> MAETRVIVVGNEKGGAGKSTIAVHLVTALLYGGAKVAVIDLDLRQRTSARFFENRRAWLDNKKIELPEPLALNLSDNDVALAERPEEEQVAGFEAAFARAMAECDFILIDTPGGDSAITRMAHGRADLVVTPMNDSFVDFDMLGTVDPVTLELTKPSLYSLTVWEGRKQRALSGQRQAMDWVVLRNRLATTE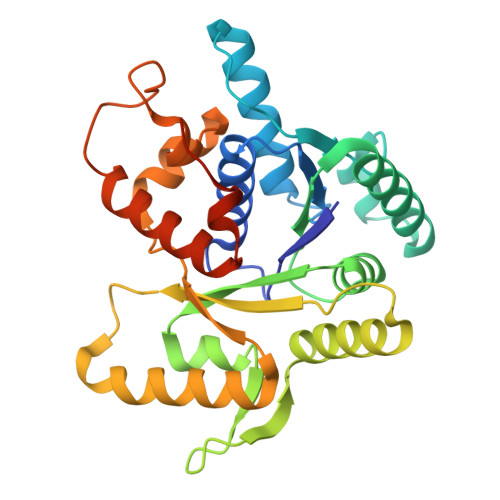ARNRKRLEDRLNALAKRVGFRIGPGLRDRVIYRELFPFGLTIADLSPQVRPVPVSLQHLAARQELRALMHSLGLSAYSGETMLAAQGSHHHHHH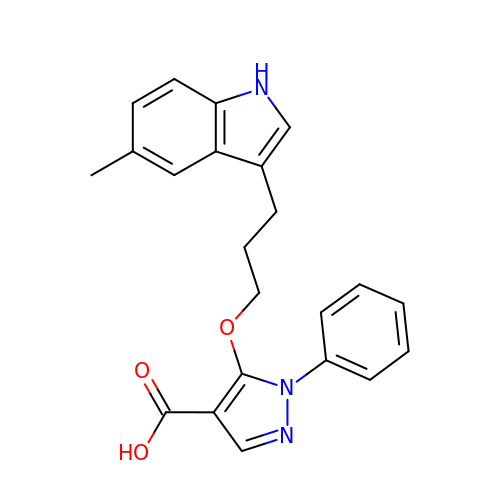5-[3-(5-methyl-1H-indol-3-yl)propoxy]-1-phenyl-1H-pyrazole-4-carboxylic acid | C22 H21 N3 O3 | MVRSNUITEJHBIY-UHFFFAOYSA-N>GSFTMNLNFSLLDEPIPLRGGTILVLEDVCVFSKIVQYCYQYEEDSELKFFDHKMKTIKESEIMLVTDILGFDVNSSTILKLIHADLESQFNEKPEVKSMIDKLVATITELIVFECLENELDLEYDEITILELIKSLGVKVETQSDTIFEKCLEILQIFKYLTKKKLLIFVNSGAFLTKDEVASLQEYISLTNLTVLFLEPRELYDFPQYILDE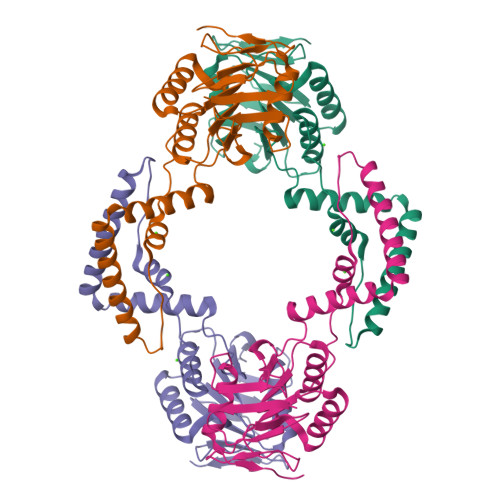DYFLITKNMV[2x]>[2x]SSLAISVANDDAGIFQPSLNALYGHPAADRGDYTAGLFLGYSHDLTDASQLSFHIAQDIYSPSGANKRKPEAVKGDRAFSAFLHTGLEWNSLATNWLRYRLGTDIGVIGPDAGGQEVQNRAHRIIGAEKYPAWQDQIENRYGYTAKGMVSLTPAIDILGVNVGFYPEVSAVGG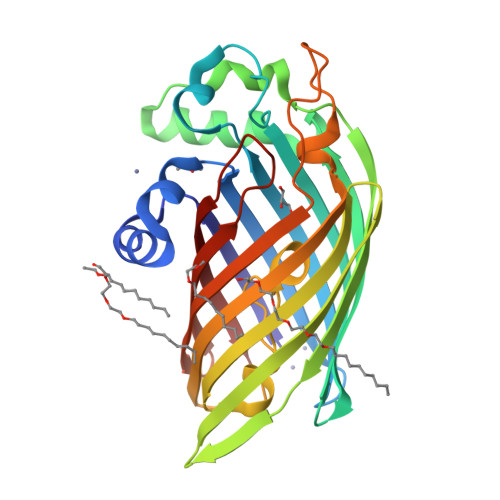NLFQYLGYGATVALGNDKTFNSDNGFGLLSRRGLIHTQKEGLIYKVFAGVERREVDKNYTLQGKTLQTKMETVDINKTVDEYRVGATIGYSPVAFSLSLNKVTSEFRTGDDYSYINGDITFFF> GEGPELHLASQFVNEACRALVFGGCVEKSSVSRNPEVPFESSAYRISASARGKELRLILSPLPGAQPQQEPLALVFRFGMSGSFQLVPREELPRHAHLRFYTAPPGPRLALCFVDIRRFGRWDLGGKWQPGRGPCVLQEYQQFRENVLRNLADKAFDRPICEALLDQRFFNGIGNYLRAEILYRLKIPPFEKARSVLEALQQHRPSPELTLSQKIRTKLQNPDLLEL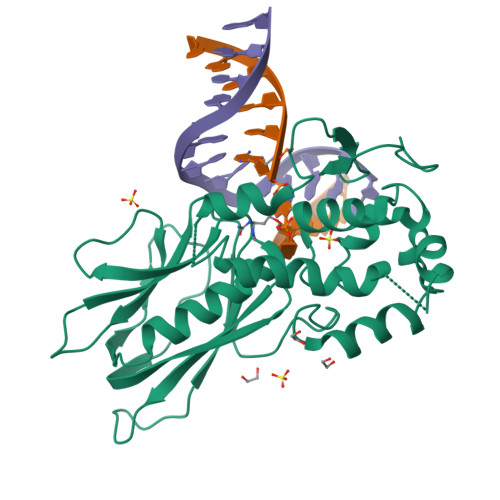CHSVPKEVVQLGGKGYGSESGEEDFAAFRAWLRCYGMPGMSSLQDRHGRTIWFQGDPGPLAPLEHHHHHH> GGGDFTTCLETESINWNCTGPFLNLGNCQKQQKKEPYTNIATQLKGLKAISVLDVPIITGIPDDIAGALRYIEEKEDFHVQLTIEYAMLSKYCDYYTQFSDNSGYSQTTWRVYLRSHDFEACILYPNQHFCRCVKNGEKCSSSNWDFANEMKDYYSGKQTKFDKDLNLALTALHHAFRGTSSAYIATMLSKKSNDDLIAYTNKIKTKFPGNALLKAIIDYIAYMKSLPGMANFKYDEFWDELLYKPNPAK

The OBV M segment encodes two glycoproteins, Gn and Gc, derived from a single polyprotein precursor, with Gn encoded upstream of Gc. Compared with other bunyaviruses, OBV Gn is relatively small, with an ectodomain of about 200 amino acids (aa), whereas Gc, with an ectodomain of ca. 900 aa long, is about twice the size of its Gc counterparts from other bunyaviruses. Our structural analysis has revealed that this region is composed of two domains: a 27 -kDa α-helical head domain and a stalk that is divided into two identically folded 19 -kDa tandem β-sandwiches. Furthermore, the head domain is well exposed to the environment and is a major target of the humoral adaptive immune system of the OBV mammalian hosts, indicating that the trigonal pyramid of the spike shields the functionally more critical membrane fusion core machinery from the host’s antibody response.

In addition to the variable region of SBV Gc, we determined the crystal structures of the Gc head domains from BUNV (aa 478–721), LACV (aa 477–722) and OROV (aa 482–702) to resolutions ranging between 2.1 Å and 2.9 Å and refined the resulting atomic models to Rfree values between 0.21 and 0.23. The aa sequence identity among the head domains of all the four viruses is low and ranges from 29% (BUNV:LACV) to 17% (SBV:BUNV). Nevertheless, they share a common tertiary structure with RMSD values between 2.0 Å over 232 Cα atoms (BUNV:LACV) and 3.7 Å over 224 Cα atoms (LACV:SBV). The head domains of BUNV, LACV, and OROV contain each a single asparagine-linked carbohydrate chain and although the positions of the respective glycosylation sites along the aa sequences are not conserved, they project from the same face of the domain carrying the two glycan chains in SBV. Nevertheless, the Gc head domains of BUNV and LACV both formed trimeric assemblies involving the same trimerization contacts in the crystals. The buried surface area at the trimer interface amounts to 1422 Å2 and 1430 Å2 on each protomer for BUNV and LACV, respectively. Whereas the atomic details at these interfaces differ between the two viruses, they comprise mainly hydrophilic residues in the region between helices h7 and h11 at the side opposite to the glycosylated surface. The concurrent observation of two very similar trimeric assemblies in two independent crystal structures strongly suggests that the trimers are physiologically relevant. The dissociation of the trimers at low pH is likely triggered by protonation of residue H590 in BUNV and in LACV, which would lead to electrostatic repulsion with positively charged side chains on the neighboring protomer. The head domain forms low-affinity trimers on the viral envelope that are recapitulated in the crystal contacts for BUNV and LACV.>[2x]GASSQRSVARMDGDVIIGALFSVHHQPPAEKVPERKCGEIREQYGIQRVEAMFHTLDKINADPVLLPNITLGSEIRDSCWHSSVALEQSIEFIRDSLISIRDEKDGINRCLPDGQSLPPGRTKKPIAGVIGPGSSSVAIQVQNLLQLFDIPQIAYSATSIDLSDKTLYKYFLRVVPSDTLQARAMLDIVKRYNWTYVSAVHTEGNYGESGMDAFKELAAQEGLCIAHSDKIYSNAGEKSFDRLLRKLRERLPKARVVVCFCEGMTVRGLLSAMRRLGVVGEFSLIGSDGWADRDEVIEGYEVEANGGITIKLQSPEVRSFDDYFLKLRLDTNTRNPWFPEFWQHRFQCRLPGHLLENPNFKRICTGNESLEENYVQDSKMGFVINAIYAMAHGLQNMHHALCPGHVGLCDAMKPIDGSKLLDFLIKSSFIGVSGEEVWFDEKGDAPGRYDIMNLQYTEANRYDYVHVGTWHEGVLNIDDYKIQMNKSGVVRSVCSEPCLKGQIKVIRKGEVSCCWICTACKENEYVQDEFTCKACDLGWWPNADLTGCEPIPVRYLEWSNIESIIAIAFSCLGILVTLFVTLIFVLYRDTPVVKSSSRELCYIILAGIFLGYVCPFTLIAKPTTTSCYLQRLLVGLSSAMCYSALVTKTNRIARILAGSKKKICTRKPRFMSAWAQVIIASILISVQLTLVVTLIIMEPPMPILSYPSIKEVYLICNTSNLGVVAPLGYNGLLIMSCTYYAFKTRNVPANFNEAKYIAFTMYTTCIIWLAFVPIYFGSNYKIITTCFAVSLSVTVALGCMFTPKMYIIIAKPERNVRSAFTTSDVVRMHVGDG

Glutamate is the main excitatory neurotransmitter in the human brain, and it exerts diverse responses through ionotropic glutamate receptors (iGluRs) and metabotropic glutamate receptors (mGluRs). mGluRs are members of the C family of GPCRs, and are divided into three groups based on G protein coupling, sequence homology, and ligand selectivity. mGlu1 and mGlu5 belong to group I and predominantly couple to Gq/11. Constitutive homo- or hetero-dimerization is the defining feature of class C GPCRs, and mGluRs form homodimers mediated by the intermolecular disulfide bond within the N-terminal extracellular domain (ECD). The large ECD of mGluRs can be divided into two parts: the venus flytrap (VFT) domain and the cysteine-rich domain (CRD). Here, we present two full-length mGlu1 structures in the apo and intermediate active states at 3.96 Å and 3.65 Å, respectively, using cryo-EM single particle analysis.

To enhance the expression and stability of mGlu1, the wild-type mGlu1 was modified by N- and C-terminal truncations and the optimized construct was expressed in the insect cell system. To seek the mGlu1 active conformation, the orthosteric agonist L-Quisqualic acid together with PAM Ro 67-4853 were added during protein purification. Eventually, we obtained the cryo-EM structure of the full-length mGlu1 homodimer at a global resolution of 3.96 Å. Although an excess amount of agonist and PAM were added during mGlu1 purification, in the cryo-EM structure, there is no electron density either for L-Quisqualic acid in the ligand binding pocket of VFTs, or for PAM Ro 67-4853 in 7TM domains, indicating that mGlu1 is in the ligand free form. In our full-length mGlu1 structure, residue Cys140 lies in the disordered region of VFTs and the disulfide bond is invisible, while the dimer interface is also formed by the B and C helices in VFTs. In addition, the distance between two lobe 2s is quite far. Therefore, the connected CRD and 7TM are also relatively far from each other. In the apo state of mGlu1, the distance between the Cα atoms of Val523-Val523 and Asn235-Asn235 from the two lobe 2s of VFTs are 60 Å and 30 Å, respectively.> MHHHHHHENLYFQGAASSHKLAEANTDFAFSLYRELAKSSPDKNIFFSPVSISSALAMLSLGAKGDTHTQILEGLGFNSEADIHQGFQHLLQTLNRPKGLQLKT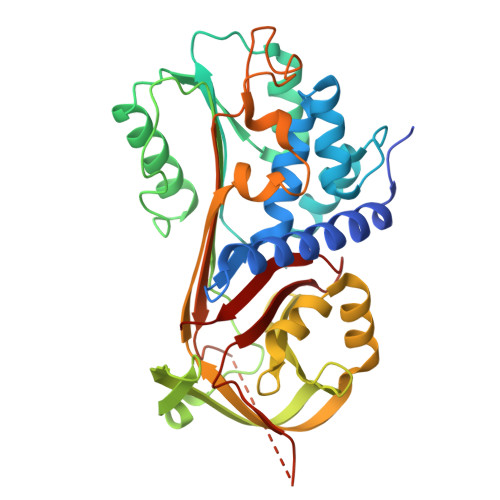ANGLFVDKSLKLLDSFLEDSKKLYQAEAFSVDFDPEEAKKQINDWVEKQTNGKIKDLLKDLDSDTVLVLVNAIYFKGKWKKPFDPENTKEEDFHVDEKTTVKVPMMSQKGKFYYYHDDELSCKVLELPYKGNASMLIILPDEGGLQHLEQSLTPETLSKWLKSLTRRSVELYLPKFKIEGTYDLKEVLSNLGITDLFSPGADLSGITEEKLYVSKAVHKAVLEVNEEGTEAAAATGVEIVPRSPPEFKADRPFLFLIRENKTGSILFMGKVVNP>MQDNTGLEELSQAQRERLAHIDFTLLFKGEAGRSYLTERFSVAPSVATQDFARYKALAPNNVMYDEKRRVHLKTSTFQPLFDYDIVRTLATISQGFGDGFLGKVRPPMACEAPF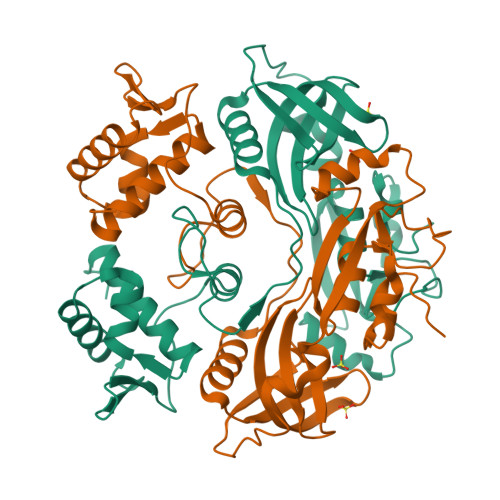HLNKPKLEVVAAISEAIHKRAVINIEYTSLSSGHGSRQIVPHTLIDNGLRWHVRAFDRKHREFRDFVLTRISEVELLEDKVNDEVETLQWDKQWNRIVELELIPHPKLAHPEAVLIDYAMENNRLRVEIRAAFAGYLLRLWNIDCSKNSKSNGREFHLALKNPEALYGVDNAALAPGYSES[8x]> MKKIIYIATIGITLLTTSCDDFLDRQVPQGIVTGDQIASPEYVDNLVISAYAIWATGDDINSSFSLWNYDV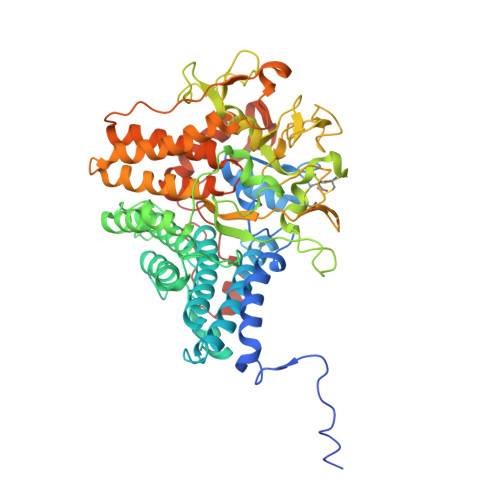RSDDCYKGGSGTEDGGVFNALEISKGINTTDWNINDIWKRLYQCITRANTALQSLDQMDEKTYPLKNQRIAEMRFLRGHAHFMLKQLFKKIVIVNDENMEPDAYNELSNTTYTNDEQWQKIADDFQFAYDNLPEVQIEKGRPAQAAAAAYLAKTYLYKAYRQDGADNALTGINEEDLKQVVKYTDPLIMAKGGYGLETDYSMNFLPQYENGAESVWAIQYSINDGTYNGNLNWGMGLTTPQILGCCDFHKPSQNLVNAFKTDSQGKPLFSTYDNENYEVATDNVDPRLFHTVGMPGFPYKYNEGYIIQKNDDWSRSKGLYGYYVSLKENVDPDCDCLKKGSYWASSLNHIVIRYADVLLMRAEALIQLNDGRITDAISLINEVRSRAAGSTMLIFNYKEDYGVNFKVTPYDLKAYAQDEAMKMLKWERRVEFGMESSRFFDLVRWGEAKDVINAYYVTEASRCSIYKNAGFTENKNEYLPVPFEQISASNGNYTQNFGWAAAAHHHHHH>MARKYFVAANWKCNGTLESIKSLTNSFNNLDFDPSKLDVVVFPVSVHYDHTRKLLQSKFSTGIQNVSKFGNGSYTGEVSAEIAKDLNIEYVIIGHFERRKYFHETDEDVREKLQASLKNNLKAVVSFGESLEQREQNKTIEVITKQVKAFVDLIDNFDNVILVYEPLWAIGTGKTATPEQAQLVHKEIRKIVKDTCGEKQAN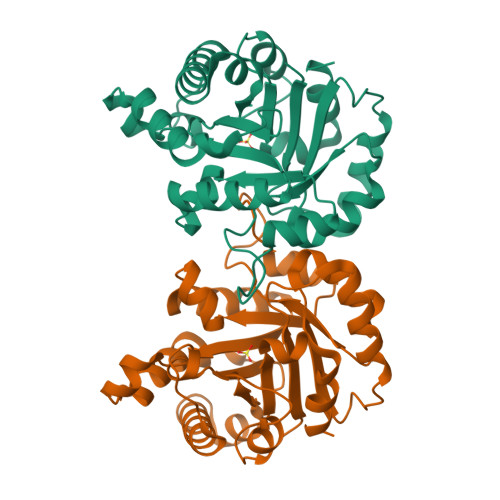QIRILYGGSVNTENCSSLIQQEDIDGFLVGNASLKESFVDIIKSAM[2x]> GPLGSERIVSLNGDITEIIFALGMGEYVVGVDSSATYPPERTKMLPNIGYQRRLSAEGILSLNPTLVIGDEAAGPPETLAQIRAAGVPLAITADPPSLDAPQQKIRFVAQALGIPQRGERLAAQVEAEIAAARDLARRITNPPHVLFLYLRGTDVQQVAGRNTAVDVMIAAAGGI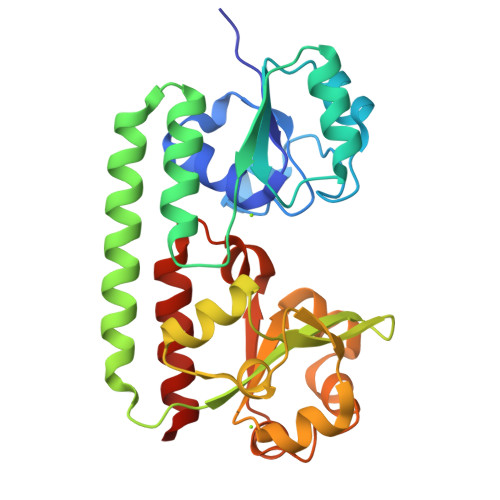NAAADAGIVEFKPLSPEVVIAAQPDVLLVLDKGLESVGGVDGLLKIPGLADTPAGRQRRIIALDDLYLLGMGPRTGQALTDLTIAFYDAAQGSRP> GMPNYKLTYFNMRGRAEIIRYIFAYLDIQYEDHRIEQADWPEIKSTLPFGKIPILEVDGLTLHQSLAIARYLTKNTDLAGNTEMEQCHVDAIVDTLDDFMSCFPWAEKKQDVKE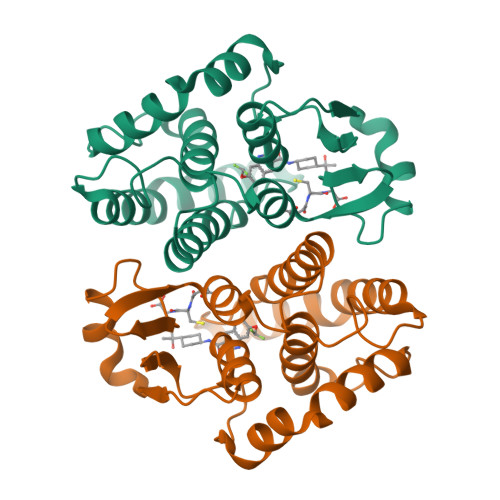QMFNELLTYNAPHLMQDLDTYLGGREWLIGNSVTWADFYWEICSTTLLVFKPDLLDNHPRLVTLRKKVQAIPAVANWIKRRPQTKL> IVGGYTCGANTVPYQVSLNSGYHFCGGSLINSQWVVSAAHCYKSGIQVRLGEDNINVVEGNEQFISASKSIVHPSYNSETYNNDIMLIKLKSAASLNSRVASISLPTSCASAGTQC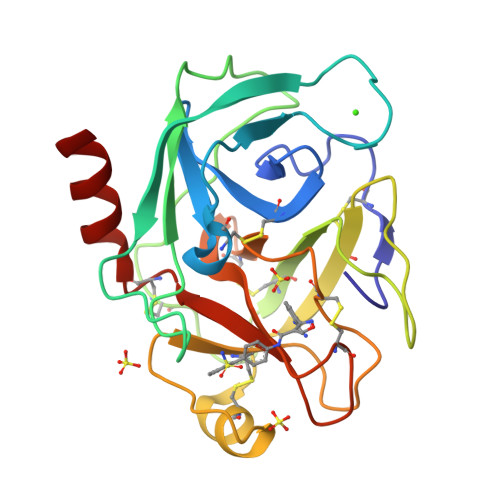LISGWGNTKSSGTSYPDVLKCLKAPILSDSSCKSASSFIITSNMFCAGYLEGGKDSCQGDSGGPVVCSGKLQGIVSWGSGCAQKNKPGFYTKVCNYVSWIKQTIASN>[2x]TYQYNMNFEKLGKCIIINNKNFDKVTGMGVRNGTDKDAEALFKCFRSLGFDVIVYNDCSCAKMQDLLKKASEEDHTNAACFACILLSHGEENVIYGKDGVTPIKDLT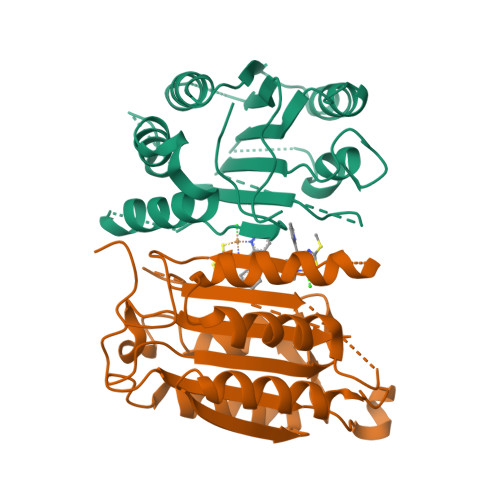AHFRGDRCKTLLEKPKLFFIQACRGTELDDGIQADSGPINDTDANPRYKIPVEADFLFAYSTVPGYYSWRSPGRGSWFVQALCSILEEHGKDLEIMQILTRVNDRVARHFESQSDDPHFHEKKQIPCVVSMLTKELYFSQ> MEHVAFGSEDIENTLAKMDDGQLDGLA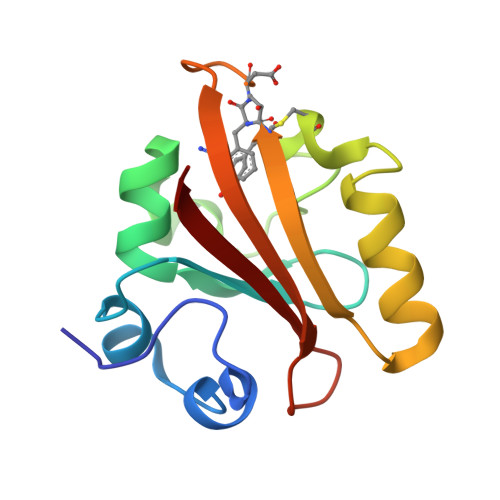FGAIQLDGDGNILQYNAAEGDITGRDPKQVIGKNFFKDVAPCTDSPEFYGKFKEGVASGNLNTMFEYTXDYQNTPTKVKVHMKKALSGDSYWVFVKRV>[6x]MSHSLREWLAFLEGKGKLKRVRKEVDPVFEIAALGKQADGICSLLFERVKGYAVPVVTGLAGDRELFAAAMSVPVEGMLEKLAAAVENPVPCRLVSPDGAPVKECIIRENIDLLKMLPIPTHHAGDAGPYITAAILIARDPDSGVRNVSIHRLQVTGPDRLGI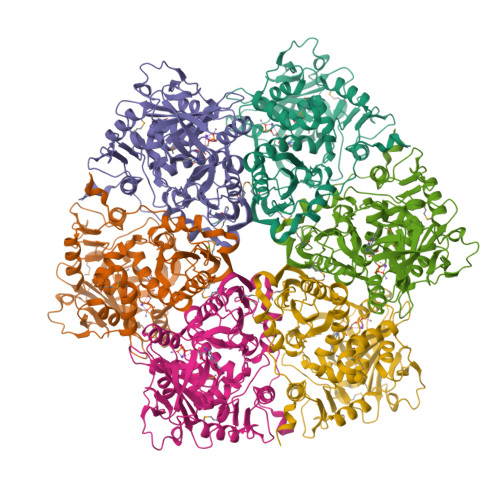LILPRHLWHFFGKAERAGRPLEIALAIGVHPAVLLASQATTRLGVDELEIASALLPQPLELVKCETVDVEVPAGAEIVIEGKILPGVREVEGPFGEYPRYYGPAAPRPVVEVTAVTHRRQPVYHTIIPASREHLLLGGIAREAVLLQTVRQAVPTVKNVHLTPGGSCRYHAVISIEKKHEGEAKNAIFAAFTSSSEVKHVVVVDHEINIFDPEEVEWAVATRCQAGRDVFIVKDAMGNRLDPSSRDGVSDKMGIDATIPLNLPGERFERISIPGLDKIKLADYLE> KKLLK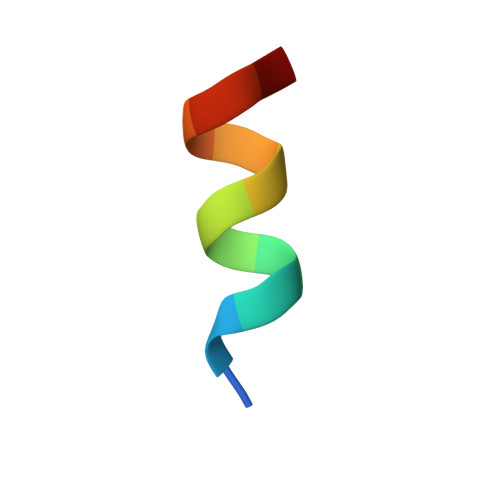LLKLLLX The enterococcal cytolysin is a two-component lanthipeptide secreted by Enterococcus faecalis that functions as a virulence factor. An extracellular protease, CylA, removes what remains of the leader peptide from CylLL’ and CylLS’ yielding mature cytolysin (CylLL” and CylLS”). CylA is a subtilisin-like serine protease that is essential for toxin activation. Like many proteases, CylA is translated as a proenzyme that undergoes activation through self-cleavage.

To afford a high-resolution structure, full-length CylA (residues Leu27-Lys412, lacking the N-terminal secretion signal sequence) with an N-terminal polyhistidine tag was expressed in E. coli, refolded from the insoluble fraction and incubated in situ to allow for autoproteolytic processing. The cleaved domains co-eluted as a single species suggesting that the pro-domain was tightly bound to the protease domain. An X-ray structure of CylA non-covalently bound to its pro-domain provided a high-resolution glimpse into substrate-enzyme interactions. The pro-domain and the catalytic domain form extensive contacts that orient the recognition sequence into the active site of the latter. Formation of the interface buries ~1270 Å2 of surface area as determined using the Proteins, Interfaces, Structures and Assemblies (PISA) server. Clear and continuous electron density is evident for the entirety of the pro-domain tail detailing interactions with the PDFKPE recognition sequence preceding the scissile bond. The side chain of Glu95 at the −1 position is within hydrogen bonding distance of the side chains of Ser260, His275 and the backbone amide of Gly262. The C-terminal carboxylate of the pro-domain is in close proximity of the hydroxy side chain of the catalytic nucleophile Ser 359. The side chain of Asn263 and the backbone amide of Thr275 are positioned to provide an oxyanion hole to stabilize the negative charge accumulated in the transition state. Notably, the −4 residue (Phe92) is directed into the catalytic domain where it is engaged in van der Waals contacts with residues in a pocket composed of Val195, Met196, Met206, and Leu225.

> MGSSHHHHHHSQDPNSLSNNISFFIDNSQTTAIEEIESELSSEKVDYIQEIGLVSFKNLDDSDRKFIGKYFNVSEGKKLPDFKPEEVNSSILNINILNKDFKSFNWPYKKILSHIDPVKEQLGKDITIALIDSGIDRLHPNLQDNNLRLKNYVNDIELDEYGHGTQVAGVIDTIAPRVNLNSYKVMDGTDGNSINMLKAIVDATNDQVDIINVSLGSYKNMEIDDERFTVEAFRKVVNYARKNNILIVASAGNESRDISTGNEKHIPGGLESVITVGATKKSGDIADYSNYGSNVSIYGPAGGYGDNYKITGQIDAREMMMTYYPTSLVSPLGKAADFPDGYTLSFGTSLATPEVSAALAAIMSKNVDNSKDSNEVLNTLFENADSFIDKNSMLKYKEVRIK Here we present four in situ and one isolated cryoEM structures of the trimeric spike of the cytoplasmic polyhedrosis virus, a member of the non-enveloped Reoviridae family and a virus historically used as a model in the discoveries of RNA transcription and capping. CPV has two functionally essential components located along the icosahedral 5-fold axis: the RNA-dependent RNA polymerase (RdRp) inside and the RNA capping turret outside;25,27 a trimeric spike is attached to the latter. Each spike monomer has four domains: N-terminal, body, claw, and C-terminal.

To determine how CPV releases new transcripts during transcription, we prepared a CPV sample treated with SAM and ATP-containing buffer (SA-CPV), which has been shown to activate the RdRP for mRNA synthesis. Serendipitously, turrets of some adjacent viral particles “kiss” one another in our structure, connecting their open ends and forming a dimer. In this dimer, there is no room for the trimeric spike to attach inside the turret; therefore, we concluded that in these structures, the trimeric spike has thoroughly detached. Comparison of sub-particle reconstructions of turrets before and after spike detachment shows that the binding of SAM and ATP to the turret protein causes global conformational changes. With these conformational changes, the diameter of the iris increases from 24 Å to 30 Å. The opening of the iris might weaken the interactions between the iris loops and the “cork” of the spike proteins, thus allowing the trimeric spike lodged in the middle of the iris to detach. The detachment of the spike clears the mRNA releasing channel and enables nascent mRNA to reach the methyltransferase (MTase) active sites and finish mRNA capping, allowing the mature mRNA to be released outside the capsid (i.e. into the cytosol). In the turreted subfamily of the Reoviridae, represented by CPV, the turret protein is a multi-functional protein: it serves as the capping enzyme, the signal sensor, and the mRNA releasing channel on the five-fold axis of the capsid. In addition, the structures of the turret vertices before and after trimeric spike detachment illustrate how the virus senses cytosolic SAM and ATP and detaches the trimeric spikes, allowing the release of newly synthesized mRNA.

>[2x]MWHYTSINNDTRVALDPKPNQIRTITKPNTVPQLGTDYLYTFNSQRRSHTLRLLGPFQYFNFSETDRGHPLFRLPLKYPSKAIPADELIDNLHSWMRSVHLLHVRSEDNTLRYNWMLGVYARSTNYTTPVGQLVVNAPAILNYSNPQDAFNSVFVALGIDYIDIPITNSNIFDDSSTPYNVRIWHAPTMTEVNHILALMRKSTLVSTHSSWHWNVLHTFHYRSESDMIDHFAAKILEDWRQKEKLDKGALVEADRVIQRLIPLSSSTYVQRLAAIGALYPNEFTENVLDLSRLSTALLQLSDTYYQHANDQLRRLYRRMYNDSRTLYMTQRHQELLLAQITADPNILLYPYTYIFTTIPTSMNYISNTGQGRIKHSLTVTGATEHDTVADIVLGQTGEDVITISMVEPMSIAVEDMYGYVLDTPTRDIWPADEQIEQKGDAVALYDTKTSRALGMFNNTVRIDDLLSPLLSLVYRTYIKGDTMTMTQGSLDHLTLCAAVDSDITFVGNRMIAPLPEGYIPKPMHRNNSTMKMLSLYVALKKLENFATNSYLMAPDTSIILLGAEREPAVNILRRFNRNVSNVRIIGMGDRAVEPNIRVRVPFPIDKNISADFIICDINSYEDQSFESMFSETISVVTTCASAATRALVKINHPSEYMINSVIERLSQLGGVFYHTALLKTASQNPYSYETYIYITPIAAAVRFPFYSNSAMINRYMTAVADDEMPIIPSIHTVIKGHSNTYSPGLFCGCVDVQSAPLALSQLKSYCSEATTWRVDSDDNLVNIIARIDPARIALEFRTRSNTSAYHEYQRYVPNGLGFKVRKTREFRYMHREVTFIHKLMMYALIREQISLTENMTQVVSIGGRNLADISVVPLNMKYVVIDPATRIETLTQEKKNIEVQSRPFQFDAANMDLENNSIYLFIAVIMNEPNGAATPARMQMDKIRNVATAMLTRTNCVAYISFYEAGIITRLDQSTAHKTIRVEEGRLKVANYVPVDTLVEADVTLMLRDIGITHEIIRPSTPELIDACSNYGIRLGSTGGAVLDVFNHYSPVIKLVRS>LMGCVAETPPRFTRTPVDQTGVSGGVASFICQATGDPRPKIVWNKKGKKVSNQRFEVIEFDDGSGSVLRIQPLRTPRDEAIYECVASNNVGEISVSTRLTVLREDQIPRGFPTIDMGPQLKVVERTRTATMLCAASGNPDPEITWFKDFLPVDTSNNNGRIKQLRSESIGGTPIRGALQIEQSEESDQGKYECVATNSAGTRYSAPANLYVRELREVRRVPPRFSIPPTNHEIMPGGSVNITCVAVGSPMPYVKWMLGAEDLTPEDDMPIGRNVLELNDVRQSANYTCVAMSTLGVIEAIAQITVKAHHHHHH[2x];>[2x]QPCPGRCICQNVAPTLTMLCAKTGLLFVPPAIDRRVVELRLTDNFIAAVRRRDFANMTSLVHLTLSRNTIGQVAAGAFADLRALRALHLDSNRLAEVRGDQLRGLGNLRHLILGNNQIRKVESAAFDAFLSTVEDLDLSYNNLEALPWEAVGQMVNLNTLTLDHNLIDHIAEGTFVQLHKLVRLDMTSNRLHKLPPDGLFLRSQGGGPKPPTPLTV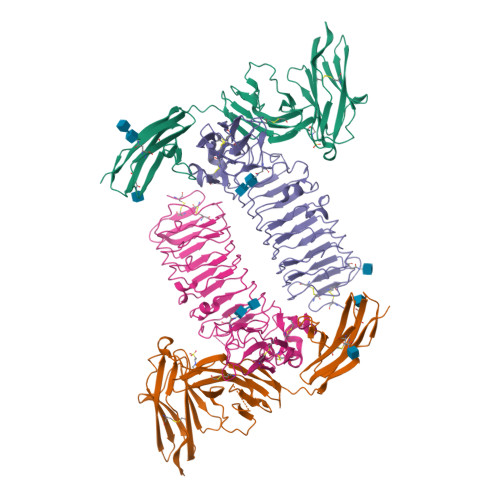SFGGNPLHCNCELLWLRRLTREDDLETCATPEHLTDRYFWSIPEEEFLCEPPLITRQAGGRALVVEGQAVSLRCRAVGDPEPVVHWVAPDGRLLGNSSRTRVRGDGTLDVTITTLRDSGTFTCIASNAAGEATAPVEVCVVPLHHHHHH>VNTIIYNVGSTTISKYATFLNDLRNEAKDPSLKCYGIPMLPNTNTNPKYVLVELQGSNKKTITLMLRRNNLYVMGYSDPFETNKCRYHIFNDISGTERQDVETTLCPNANSRVSKNINFDSRYPTLESKAGVKSRSQVQLGIQILDSNIGKISGVMSFTEKTEAEFLLVAIQMVSEAARFKYIENQVKTNFNRAFNPNPKVLNLQETWGKISTAIHDAKNGVLPKPLELVDASGA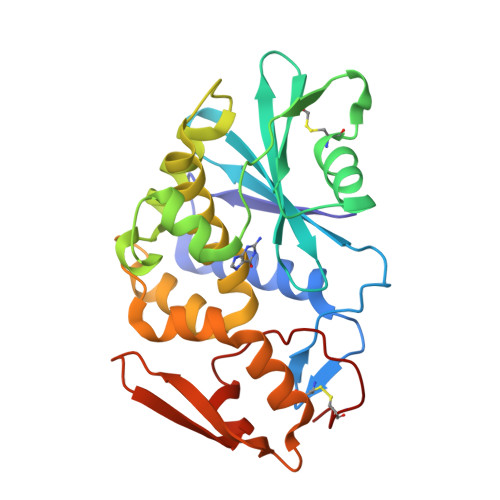KWIVLRVDEIKPDVALLNYVGGSCQTT[2x]In some pathogenic microbes, the response to oxidative stress is controlled by a SirTM/zinc-containing macrodomain (Zn-Macro) pair responsible for establishment and removal of the modification, respectively. Strikingly, however, the “catalytic loop” found in all other MacroD-type enzymes (also termed “loop 1”) is replaced with and extended loop containing the zinc-coordinating Cx(4)HxC motif, here termed the Zn-loop. To gain a closer understanding of the functional role of the 3α-bundle and coordinated Zn2+ ion, we solved structures from the three sub-branches of Zn-Macros namely from S. aureus (SauMacro), Methanobrevibacter oralis (MorMacro), and macrodomain-fused SirTM protein (Mfs1) from Fusarium oxysporum f.sp. cubense race 1 (Foc1Mfs1) in their apo form as well as of S. pyogenes (SpyMacro) and MorMacro bound to ADP-ribose (ADPr). In all structures, the Zn2+ ion is tetrahedrally coordinated with three metal-coordination residues within the Zn-loop, while the fourth coordination-contact is exchangeable and is provided by either ADPr, a water molecule, or a symmetry-related protomer within the crystal.

Given the intrinsic linkage between Zn2+ ion coordination and catalytic activity, we were unable to crystallize our protein with Asp-ADPr–modified GcvH-L or a peptide containing the modification. Therefore, we synthesized asparagine-ADP-ribose (Asn-ADPr) as close, nonhydrolyzable isostere for structural studies. Having synthesized Asn-ADPr, we were able to crystallize the MorMacro:Asn-ADPr complex. The overall structure closely resembles the ADPr-bound form (RMSD 0.515 Å over 245 Cα). The ADPr moiety placement is isostructural to our SpyMacro:ADPr complex with zinc(II) contact made by the Nδ2 atom of the modified Asn side chain, which again leads to a tetrahedral coordination of the Zn2+ ion. We could observe an isostructural water molecule in our structures of SpyMacro and MorMacro in complex with ADPr and Asn-ADPr, respectively, thus suggesting that the Pα phosphate group could act as Lewis base in the reaction. Moreover, the C1’’ centre appears to be strongly positively polarized due to the direct substrate coordination by the Zn2+ ion as well as the coordination of the 2’’ OH group by a conserved histidine-aspartate dyad (Asp116 and His120 in MorMacro).

>[3x]GPMNNDEQLEFLINYLLDERSESIDIPKTFSEKRNLLRSLMNMRHPSNISEEFLRIQDEFLSRETANKNLTSVEDISLSSGKIMLWQGDITTLSADAIVNAANSKLLGCFIPMHNCIDNIIHSASGLQLREECNRMIMLQGGDEDVGKAKITNAYNLPSKYVVHTVGPSIERGMRVSSDDVKKLERCYNSCLELASEYKLNSIAFCCISTGVFNFPQKKAAEIAIRTVKDFLNSNETSLNHIIFDVFTDKDYDIYKKLLFGN> AGSGHMDPDFLYRWALIGLAAFGAFSFATLFFVPAPYGRHQRGGWGPTVPTRLAWIAQELPAPLVFALVFARGEHADRLVPLLLLGLWQLHYLQRTFVFPLLMRVGAKRTPLVTALLAFVFNCVNGAANAYAITHGALRHTEAWLADPRFAIGALLFLGGWALNLHSDAILRRLRAPGETRYEIPRGGAYRLVSCPNYLGEIVEWCGWALATWTYAGAVFAFFTFANLFPRALAHHRWYRERFPDYPRERKAVIPFVV

Enzymes of steroid 5α-reductase family, which catalyze the 3-oxo-Δ4 reduction reactions, have critical roles in steroidogenesis. SRD5A1 and -2 are mainly involved in the metabolism of steroid hormones, whereas SRD5A3 converts polyprenol into dolichol for the early steps of protein N-linked glycosylation. Both SRD5A1 and -2 are endoplasmic reticulum membrane-embedded and utilize NADPH as a hydride (H−) donor for the Δ4 reduction reactions. In this work, we report the crystal structure of PbSRD5A from Proteobacteria bacterium and homology-based structural models of human HsSRD5A1 and -2. PbSRD5A shared 60.6% and 51.5% sequence similarities with HsSRD5A1 and -2, respectively.

After extensive crystallization trails, the crystals of PbSRD5A in space group C2221 yielded in several conditions under monoolein lipid using lipidic cubic phase crystallization method and diffracted x-ray to 2.0 Å resolution. PbSRD5A comprises seven transmembrane segments (TMs), with the N-termini located on the periplasmic side of the plasma membrane and C-termini on the cytosolic side. The connecting sequence between TM1 and TM2 adapted a short β strand (β1–2), which formed antiparallel β-sheets with the corresponding strand β3-4 linking TM3 and TM4. With most amino acids assigned in the electron density map, two omitted electron densities were clearly visible in the central cavity near the cytoplasmic side. NADPH perfectly fitted into one of the densities mainly coordinated by TM5-7 of PbSRD5A. NADPH formed extensive hydrogen bonds with N159, D163, and R170 on TM5, N192, Y193, and E196 on TM6, and T219, N222, R226, and H230 on TM7. The other elongated strip density was modeled with the crystallization lipid monoolein, whose alkenyl “tail” is accommodated well in the hydrophobic pocket majorly composed by the residues located on TM1-4. Considering of the hydrophobicity of steroid substrates and the orientation of NADPH, more specifically the position of nicotinamide, we hypothesized that monoolein probably occupied the steroid substrates binding pocket. In the substrate-free PbSRD5A structure, Y87 donates a hydrogen bond to a water molecule, which in turn hydrogen bonded with E54. Intriguingly, the movements of TM1s, combined with the observation of significantly large B factor value of TM1 in PbSRD5A structure, suggested that the TM1 may play important roles in the substrate entering and releasing.>[6x]MSKYVDRVIAEVEKKYADEPEFVQTVEEVLSSLGPVVDAHPEYEEVALLERMVIPERVIEFRVPWEDDNGKVHVNTGYRVQFNGAIGPYKGGLRFAPSVNLSIMKFLGFEQAFKDSLTTLPMGGAKGGSDFDPNGKSDREVMRFCQAFMTELYRHIGPDIDVPAGDLGVGAREIGYMYGQYRKIVGGFYNGVLTGKARSFGGSLIRPEATGYGLVYFTEAMLKRHGMGFEGMRVSVSGSGNVA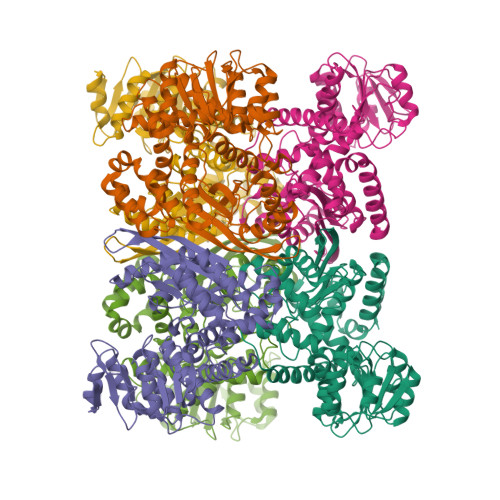QYAIEKAMEFGARVITASDSSGTVVDESGFTKEKLARLIEIKASRDGRVADYAKEFGLVYLEGQQPWSLPVDIALPCATQNELDVDAAHQLIANGVKAVAEGANMPTTIEATELFQQAGVLFAPGKAANAGGVATSGLEMAQNAARLGWKAEKVDARLHHIMTDIHDGSAAAAERYGLGYNLVAGANIVGFQKIADAMMAQGIAW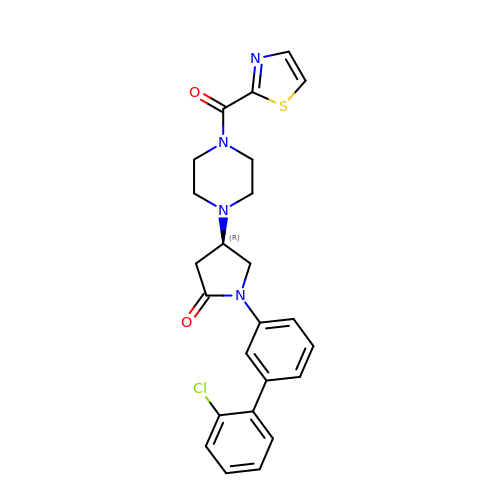(4R)-1-(2'-chloro[1,1'-biphenyl]-3-yl)-4-[4-(1,3-thiazole-2-carbonyl)piperazin-1-yl]pyrrolidin-2-one | C24 H23 Cl N4 O2 S | OFKDHTKARMXLGB-LJQANCHMSA-N>MS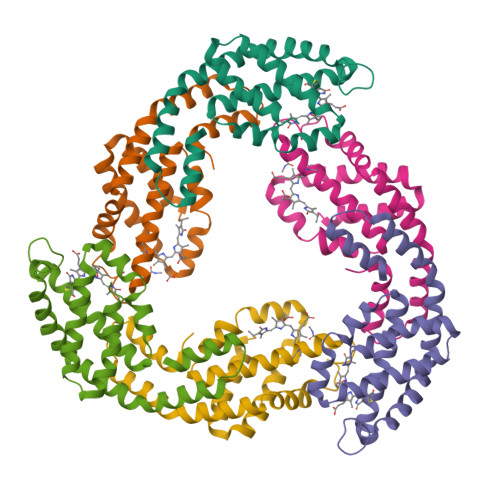VVTKSIVNADAEARYLSPGELDRIKNFVSTGERRLRIAQTLTENRERIVKQAGDQLFQKRPDVVSPGGNAYGEEMTATCLRDLDYYLRLVTYGIVAGDVTPIEEIGLVGVREMYNSLGTPIPAVAEGIRAMKNVACSLLSAEDAAEAGSYFDFVIGAMQ[4x];>MQDAITAVINASDVQGKYLDTAAMEKLKAYFATGELRVRAASVISANAANIVKEAVAKSLLYSDITRPGGNMYTTRRYAACIRDLDYYLRYATYAMLAGDPSILDERVLNGLKETYNSLGVPIAATVQAIQAMKEVTASLVGADAGKEMGIYFDYICSGLS[4x]> MFERFTDRARRVVVLAQEEARMLNHNYIGTEHILLGLIHEGEGVAAKSLESLGISLEGVRSQVEEIIGQGQQAPSGHIPFTPRAKKVLELS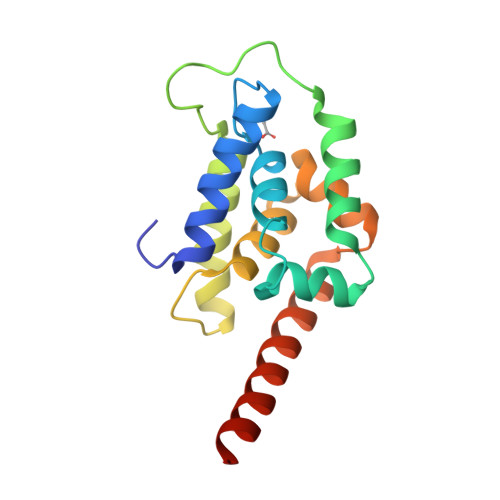SREAPQLGHNYIGTEHILLGLIREGEGVAAQVLVKLGAELTRVRQQVIQLLSGYKLAAALEHHHHHH>MSLSKKRKLESGDSGGAGAGGEGAEEENGGEQEAAPPRPRRTKSERDQLYYECYSDVSVHEEMIADQVRTEAYRLGILKNWAALRGKTVLDVGAGTGILSIFCAQAGARRVYAVEASAIWQQAREVVRLNGLEDRVHVLPGPVETVELPERVDAIVSEWMGYGLLHESMLSSVLHARTKWLKEGGLLLPASAELFVAPISDQMLEWRLGFWSQVKQHYGVDMSCMESFATRCLMGHSEIVVQDLSGEDVLARPQRFAQLELARAGLEQELEAGVGGRFRCSCYGSAPLHGFAVWFQVTFPGGDSEKPLVLSTSPLHP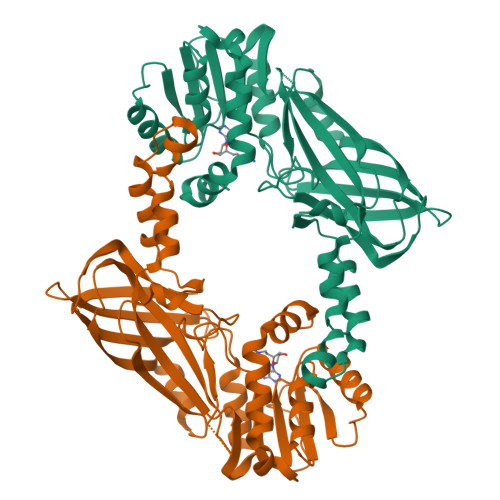ATHWKQALLYLNEPVPVEQDTDISGEITLLPSPDNPRRLRILLRYKVGDHEEKTKDFAMEDGSENLYFQ[2x]> EAIVGKVTEVNKDTFWPIVKAAGDKPVVLDMFTQWCGPSKAMAPKYEKLAEEYLDVIFLKL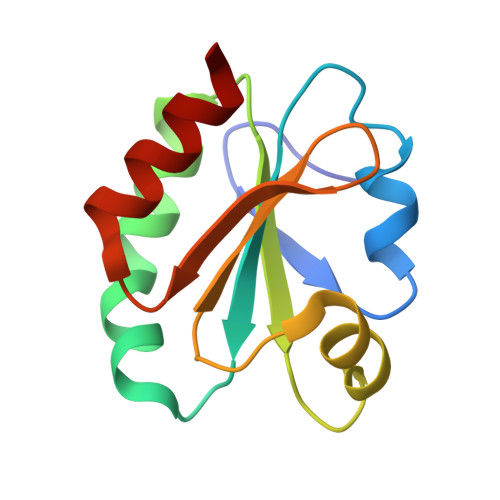DCNQENKTLAKELGIRVVPTFKILKENSVVGEVTGAKYDKLLEAIQAARS> NDDKIVVCYYGTWATYRTGLGKFDVDDIDPFLCTHLVYAFIGINAEGTALALDPELDVERGNFKQFTSLKEKNPNLKTLVAVGGWSEGSAQYSIMAAEPEYRQNFIQTSLAMIL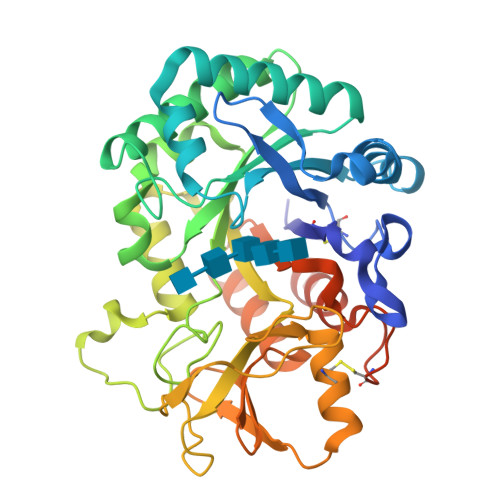EYNFDGLDVDWLYPNRRDTVHGEDDIEQFSTLLKELREEFDNYGLLLTVAVSAVEEAAVQSYDVPSVAKYVDYIGVMTYDMHGAWDSVTGHNAPLFISEGESAEQESTLYNVNNAVQYWLSAGCPPEKLVMGVPFYGRTFQLSDPSVNAPNSPSNGAGLAGPYTAESGYVGYNEFCYILQQESSWTVQTDNLAKVPYAFLDYNWVSFDNVESMTAKVEYANSFNLRGIMLWSIETDDFHGLCGEGTFPLLNTINTVLAEGSTEARHNNPPGHHHHHHHH> EVPIVTRAEWNAKPPNGAIDSMVTPLPRAVIAHTAGGACADDVTCSQHMRNLQNFQMSKQKFSDIGYHYLIGGNGKVYEGRSPSQRGAFAGPNNDGSLGIAFIGNFEERAPN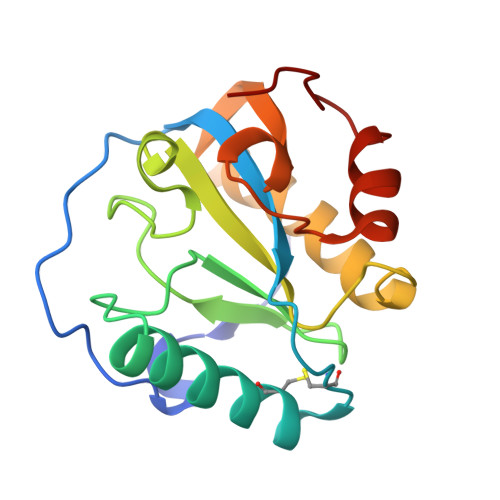KEALDAAKELLEQAVKQAQLVEGYKLLGHRQVSATKSPGEALYALIQQWPNWSEEML>[12x]MGHHHHHHQKNPISPTIPLDRDGVFHGFLKLPHSRDD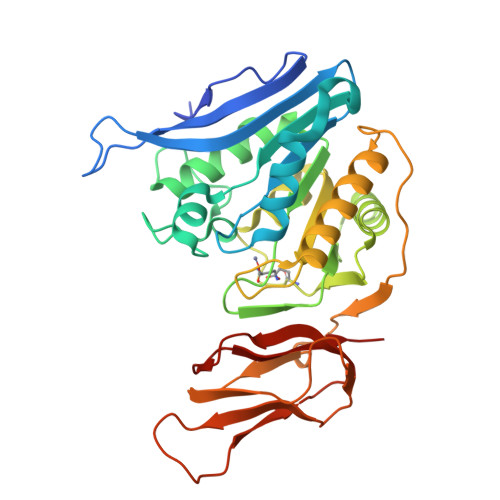SAWGSVMIPLTVIKNGAGPTALLTGANHGDEYEGPVALHELAATTSAEDVTGRLIIVPAFNYPAFRAGSRTSPIDRGNLNRSFPGRPDGTVTEKIADYFQRTLLPMADLAVDFHSGGKTLDFVPFAAAHILEDKATQAACFAAMKAFNAPYSVELLEIDSAGMYDTAVEEMGKVLVTTELGGGGSSSARSNAIAKKGLRNVLIHAGILKGEMQLDETVNLTMPDDDCFVFSEGDGLFEMMIDLGAPVAKGDLLARVWPLDRTGQPPVEYRARRAGLVISRHFPGLIKSGDCVAVVGVTGA> MVRKMRIAVIDYDKCNPDKCGHFLCERVCPVNRMGGEAIIIDEENYKPIIQEASCTGCGICVHKCPFNAISIVNLPEQLDEDCVHRYGVNAFVLYRLPIVKDGMVVGIVGPNGTGKTTAVKILAGQLIPNLCEDNDSWDNVIRAFRGNELQNYFERLKNGEIRPVVKPQYVDLLPKAVKGKVRELLKKVDEVGKFEEVVKELELENVLDRELHQLSGGELQRVAIAAALLRKAHFYFFDEPSSYLDIRQRLKVARVIRRLANEGKAVLVVEHDLAVLDYLSDVIHVVYGEPGVYGIFSKPKGTRNGINEFLQGYLKDENVRFRPYEIRFTKLSERVDVERETLVEYPRLVKDYGSFKLEVEPGEIRKGEVIGIVGPNGIGKTTFVKMLAGVEEPTEGKVEWDLTVAYKPQYIKAEYEGTVYELLSKIDSSKLNSNFYKTELLKPLGIIDLYDRNVEDLSGGELQRVAIAATLLRDADIYLLDEPSAYLDVEQRLAVSRAIRHLMEKNEKTALVVEHDVLMIDYVSDRLIVFEGE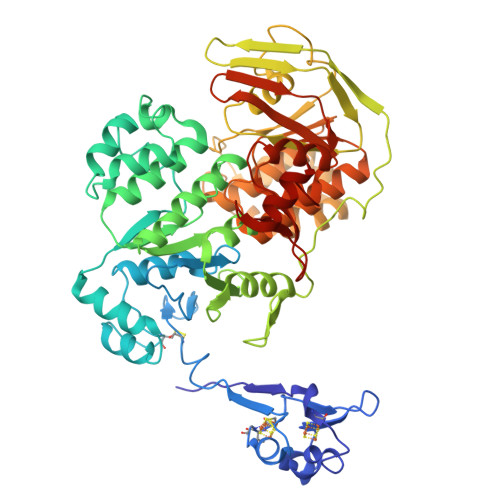PGRHGRALPPMGMREGMNRFLASVGITFRRDPDSGRPRANKEGSVKDREQKARGEYYYA O-[(2R,3S,4R,5R)-5-(2-amino-6-oxo-3,6-dihydro-9H-purin-9-yl)-2-({[(S)-({(2R,3S,4R,5R)-5-(2,4-dioxo-3,4-dihydropyrimidin-1(2H)-yl)-4-hydroxy-2-[(thiophosphonooxy)methyl]tetrahydrofuran-3-yl}oxy)(sulfanyl)phosphoryl]oxy}methyl)-4-hydroxytetrahydrofuran-3-yl] 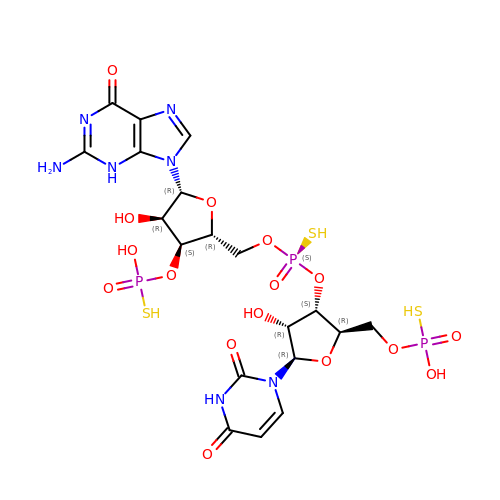dihydrogen (S)-phosphorothioate | C19 H26 N7 O16 P3 S3 | PRHQISJBVGJFKN-VXGQQCRQSA-N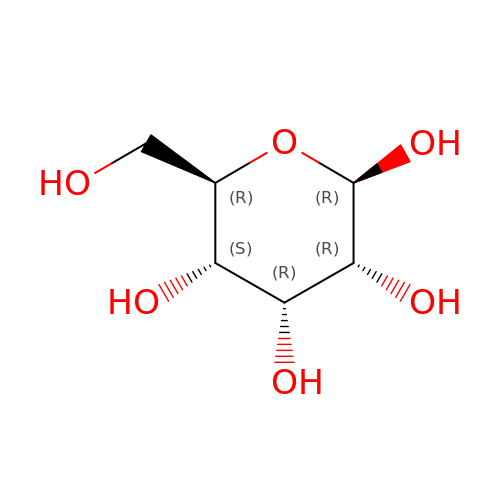beta-D-allopyranose | C6 H12 O6 | WQZGKKKJIJFFOK-QZABAPFNSA-N>AEETCFDKYTGNTYRVGDTYERPKDSMIWDCTCIGAGRGRISCTIANRCHEGGQSYKIGDTWRRPHETGGYMLECVC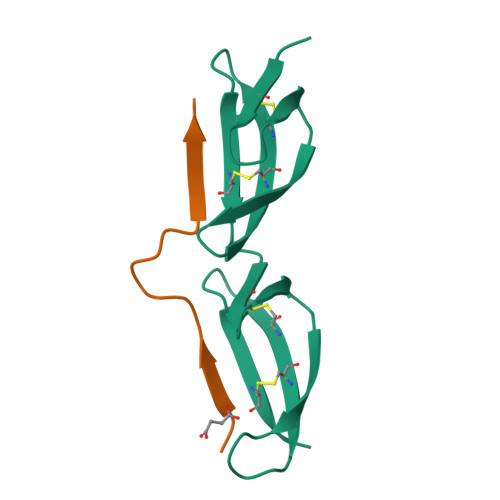LGNGKGEWTCKPI[6x];>XETLTGQYDKNLVTTVEEEYDSX[6x]>MHHHH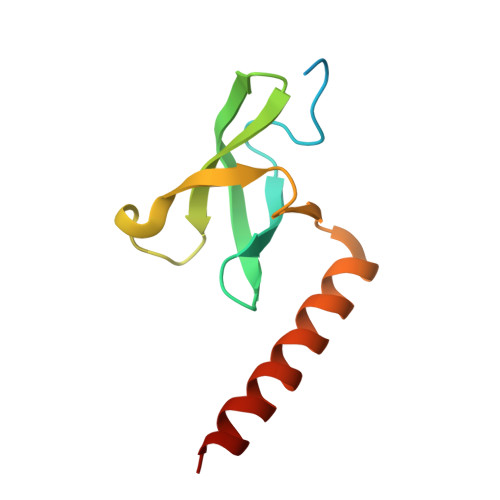HHAMGILMAPKQDPKPKFQEGERVLCFHGPLLYEAKCVKVAIKDKQVKYFIHYSGWNKNWDEWVPESRVLKYVDTNLQKQRELQKANQEQYAEGKMR[6x]> AAGCGCCUGGACUUAAAGCCAUUGCACU;> CCGGCUUUAAGUUGACGAGAGCAGGGUUUAUCGAGACAUCGGCGGGUGCCCUGCGGUCUUCCUGCGACCGUUAGAGGACUGGUAAAACCACAGGCGACUGUGGCAUAGAGCAGUCCG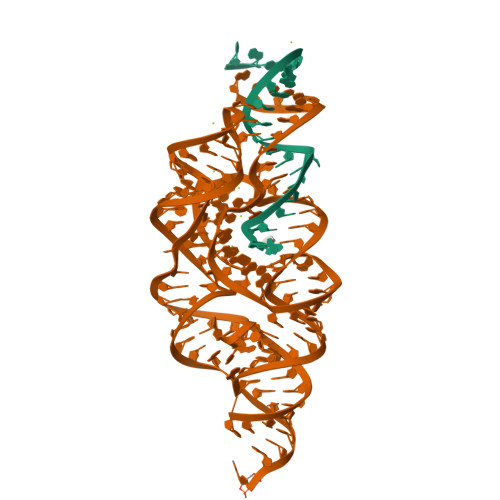GGCAGGAA>[4x]AVPMDTISGPWGNNGGNFWSFRPVNKINQIVISYGGGGNNPIALTFSSTKADGSKDTITVGGGGPDSITGTEMVNIGTDEYLTGISGTFGIYL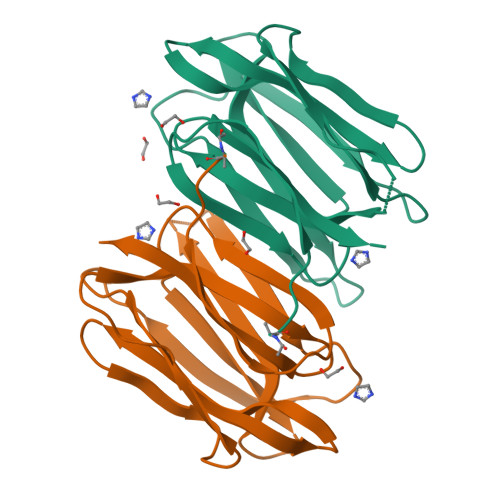DNNVLRSITFTTNLKAHGPYGQKVGTPFSSANVVGNEIVGFLGRSGYYVDAIGTYNRHK N-[1-(3-chlorophenyl)-3-methyl-1H-pyrazol-5-yl]pyrazolo[1,5-a]pyrimidine-3-carboxamide 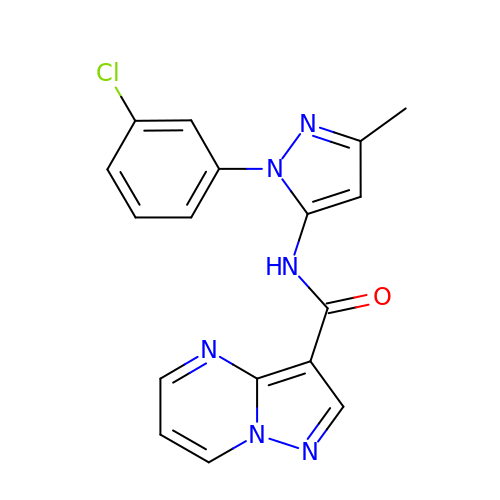| C17 H13 Cl N6 O | YLBXBHSEZZNJPX-UHFFFAOYSA-N>[2x]SKPFTLPILTLGELTNSRFPLPIDVLYTNPNESAIVQCQNGRCTLDGELQGTTQLLPTGICAFRGKVTQQVQDEHRGTHWNMTVTNLNGTPFDPTEDVPAPLGTPDFSGQIYGVISQRNTNTVPGEGNLPANRAHEAVIATYSPKFTPKLG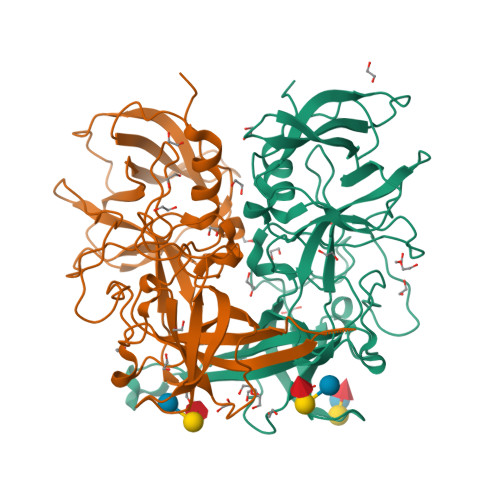NIQFSTWETQDVSSGQPTKFTPVGLASVDANSHFDQWTLPSYSGALTLNMNLAPSVAPVFPGECLLFFRSFIPLKGGYGNPAIDCLMPQEWVQHLYQESAPSLSDVALVRYVNPETGRTLFEAKLHRNGFLTVARNSAGPVVAPTNGYFRFDSWVNQFYTLAPM>[2x]MGRDHRKIGKQLDLYHMQEEAPGMVFWHNDGWTIF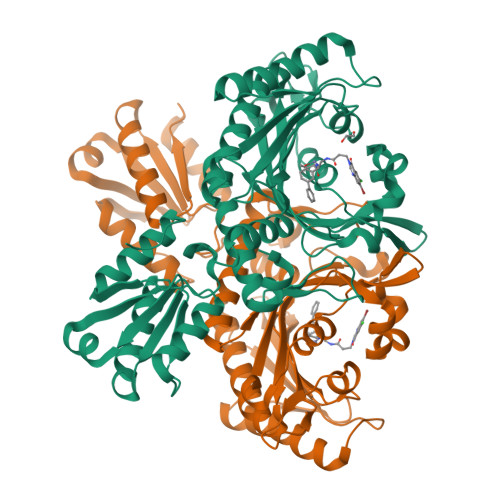RELEVFVRSKLKEYQYQEVKGPFMMDRVLWEKTGHWDNYKDAMFTTSSENREYCIKPMNCPGHVQIFNQGLKSYRDLPLRMAEFGSCHRNEPSGALHGLMRVRGFTQDDAHIFCTEEQIRDEVNACIRMVYDMYSTFGFEKIVVKLSTRPDKRIGSDEMWDRAEADLAVALEENNIPFEYQLGEGAFYGPKIEFTLYDCLDRAWQCGTVQLDFSLPSRLSASYVGEDNERKVPVMIHRAILGSMERFIGILTEEFAGFFPTWLAPVQVVVMNITDSQSEYVNELTQKLQNAGIRVKADLRNEKIGFKIREHTLRRVPYMLVCGDKEVEAGKVAVRTRRGKDLGSLDVNDVIEKLQQEIRSRSLQQLEELEHHHHHH>[2x]GAMASAQQTKQDEANRLSRDYVAGVNFLLSNQQDKAVDLFLDMLKEDTGTVEAHLTLGNLFRSRGEVDRAIRIHQTLMESASLTYEQRLLAVQQLGRDYMAAGLYDRAEDMFNQLTDETEFRVGALQQLLQIYQLTSDWQKAIEVAERLVKLGKDKQRIEIAHFYCELALQQMGNDDMDRAMALLKKGAAADKNSARVSIMMGRVYMARGDYAKAVESLQRVIVQDKELV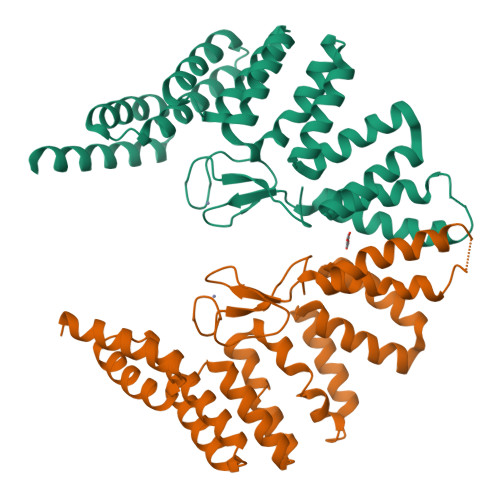SETLEMLQTCYQQLGKNAEWAEFLRRAVEENTGAGAELMLADILEAREGSDAAQVYITRQLQRHPTMRVFHKLMDYHLNEAEEGRAKESLMVLRDMVGEQVRSKPRYRCQKCGFTAYTLYWHCPSCRAWSTIKPIRGLDGQ> MAEYPLPKFHFQVDWGGSRLGFTEVSGLDVETEVIEYREGNLP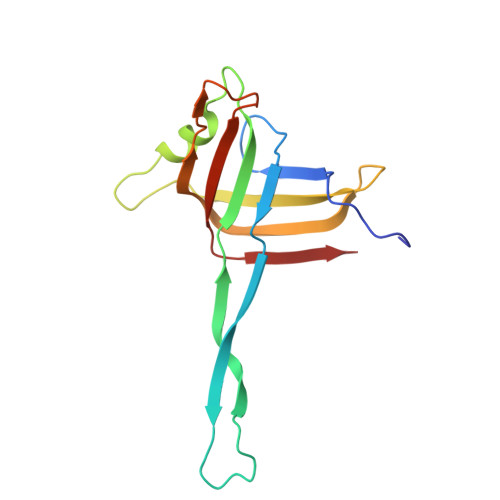QYHKLKMPGMQKFSNITMKRGTFQGDNDFYKWWNTVALNTIERRDLTISLLNEKHEPVVVWKVNRAWPTKVQSTDLKGDGNEVAIESIEVAHEGLTIQNG>[2x]RNLMIVDGTNLGFRFKHNNSKKPFASSYVSTIQSLAKSYSARTTIVLGDKGKSVFRLEHLPEYKGNRDEKYAQRTEEEKALDEQFFEYLKDAFELCKTTFPTFTIRGVEADDMAAYIVKLIGHLYDHVWLISTKGDWDTLLTDKVSRFS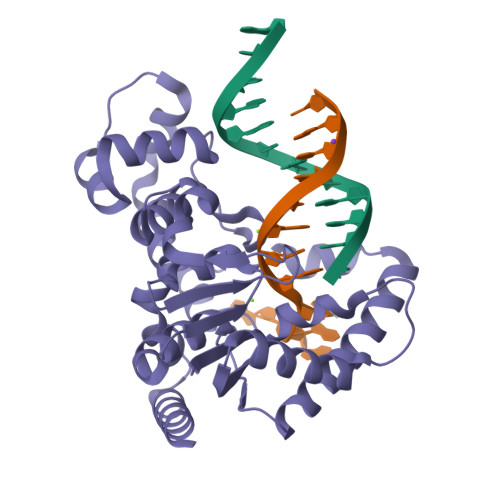FTTRREYHLRDMYEHHNVDDVEQFISLKAIMGDLGDNIRGVEGIGAKRGYNIIREFGNVLDIIDQLPLPGKQKYIQNLNASEELLFRNLILVDLPTYCVDAIAAVGQDVLDKFTKDILEIAEQ> ETDKNISEAFEDLSKLMIKAKEM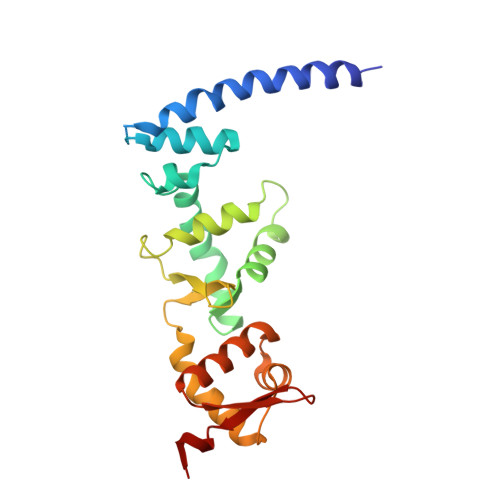VELSKSIANKIKDKQGDITEDETIRFKSYLLSMGIANPVTRETYGSGTQYHMQLAKQLAGILQVPLEERGGIMSLTEVYCLVNRARGMELLSPEDLVNACKMLEALKLPLRLRVFDSGVMVIELQSHKEEEMVASALETVSEKGSLTSEEFAKLVGMSVLLAKERLLLAEKMGHLCRDDSVEGLRFYPNLFMTQS>MKFETQLIHGGISEDATTGATSVPIYMASTFRQTKIGQNQYEYSRTGNPTRAAVEALIATLEHGSAGFAFASGSAAINTVFSLFSAGDHIIVGNDVY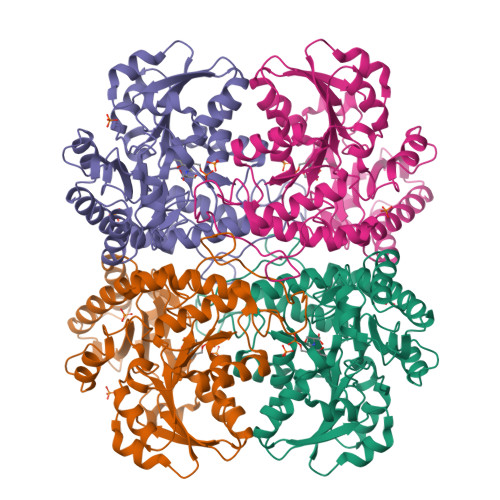GGTFRLIDAVLKHFGMTFTAVDTRDLAAVEAAITPTTKAIYLETPTNPLLHITDIAAIAKLAQAHDLLSIIDNTFASPYVQKPLDLGVDIVLHSASAYLGGHSDVIGGLVVTKTPALGEKIGYLQNAIGSILAPQESWLLQRGMKTLALRMQAHLNNAAKIFTYLKSHPAVTKIYYPGDPDNPDFSIAKQQMNGFGAMISFELQPGMNPQTFVEHLQVITLAESLGALESLIEIPALMTHGAIPRTIRLQNGIKDELIRLSVGVEASDDLLADLERGFASIQADLEHHHHHH[6x]>MEQPGELVGRALVIVVDDRTAHGEEDHSGPLVTELLGEAGFVVDGVVVVASDEVEIRNALNTAVIGGVDLVVSVGGTGVTPRDVTPEATRELLDRELLGISEALRASGLAAGIVDAGLSRGLAGISGSTLVVNIAGSRAAVRDGMATLGPL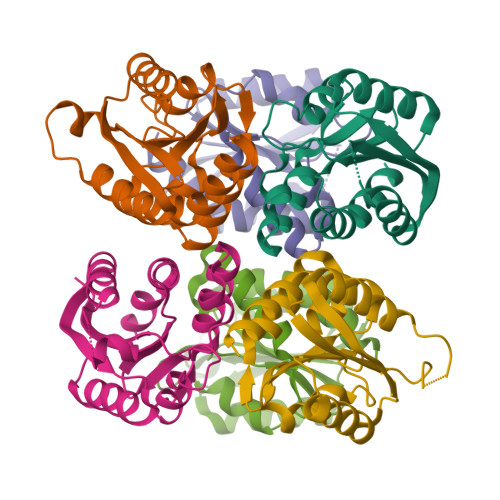AVQIIGQLSSLEILEHHHHHH[6x]WD40 proteins are a subfamily of propeller proteins with no intrinsic enzymatic activity, but their stable, modular architecture and versatile surface have allowed evolution to adapt them to many vital roles. By computationally reverse-engineering the duplication, fusion and diversification events in the evolutionary history of a WD40 protein, a perfectly symmetrical homologue called Tako8 was made. A different computational approach was employed to redesign Tako8 to create Ika8, a fourfold-symmetrical protein in which neighbouring blades carry compensating charges. Tako and Ika are the first successfully designed eight-bladed WD40-repeat proteins for which structures have been confirmed crystallographically.

The entire protein is well represented in the electron-density map. The eightfold symmetry of the protein is reflected in the water structure within the central cavity, which is 11 Å across. The tetragonal crystals show large solvent channels, and the monomeric form shows a pseudo-cubic arrangement of molecules around large symmetrical cavities. In both crystal forms the Tako8 molecules show a conserved interaction at the top side where two proteins meet face to face. The crystal-packing interaction is mediated by a hydrogen-bonding pattern with eightfold symmetry. The difference between the two crystal forms arises from different water-mediated interactions at the outer rim of the toroid. The individual repeats of the Tako8 protein can be perfectly aligned. Tako8 was found to have highest stability around pH 8, but to be extremely unstable in the absence of salt.

> GSHMGQSLRTLQGHQSAVTSLQFNDNIVVSGSDDSTVKVWDIKTGQSLRTLQGHQSAVTSLQFNDNIVVSGSDDSTVKVWDIKTGQSLRTLQGHQSAVTSLQFNDNIVVSGSDDSTVKVWDIKTGQSLRTLQGHQSAVTSLQFNDNIVVSGSDDSTVKVWDIKTGQSLRTLQGHQSAVTSLQFNDNIVVSGSDDSTVKVWDIKTGQSLRTLQGHQSAVTSLQFNDNIVVSGSDDSTVKVWDIKTGQSLRTLQGHQSAVTSLQFNDNIVVSGSDDSTVKVWDIKTGQSLRTLQGHQSAVTSLQFNDNIVVSGSDDSTVKVWDIKGS[2,3-bis(oxidanyl)phenyl]-[6-(2-fluoranyl-3-oxidanyl-phenyl)pyridin-2-yl]methanone | C18 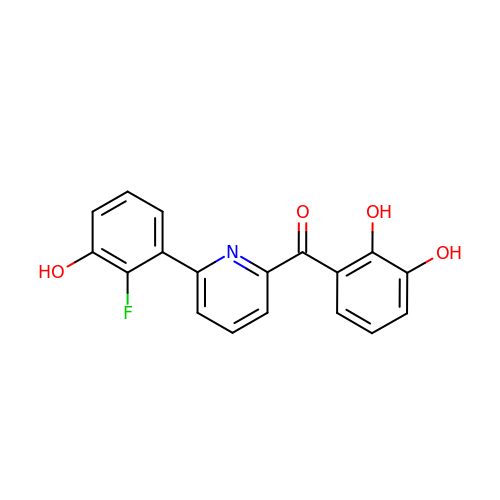H12 F N O4 | OESDFRIOBRBPRO-UHFFFAOYSA-N(2R)-N~8~-HYDROXY-2-{[(5-METHOXY-2-METHYL-1H-INDOL-3-YL)ACETYL]AMINO}-N~1~-[2-(2-PHENYL-1H-INDOL-3-YL)ETHYL]OCTANEDIAMIDE 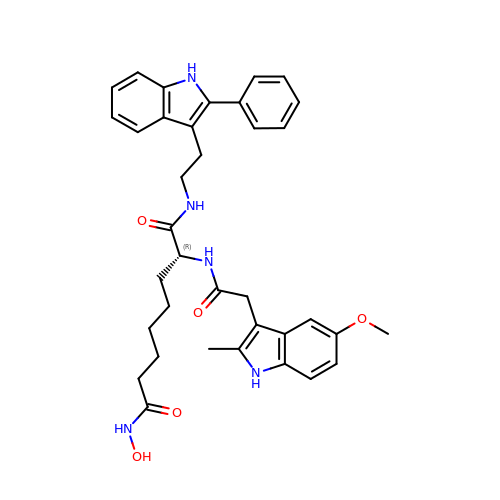| C36 H41 N5 O5 | VBWCMILVHANAGG-JGCGQSQUSA-N>MKKIEHKMVAVNGLNMHLAELGEGPTILFIHGFPELWYSWRHQMVYLAERGYRAVAPDLRGYGDTTGAPLNDPSKFSILHLVGDVVALLEAIALNEEKVFVVAHDLGAYIAWHLCLFRPDKVKALVNLSVHFSKRNPKMNKVEGLKAIYGEDHYVSRFQVPGEIEAEFAPIGAKSVLKKILTYR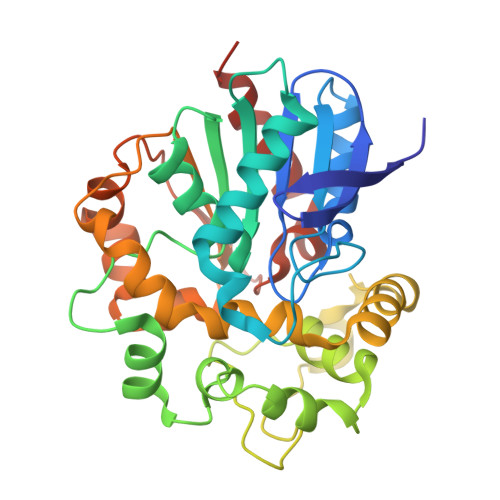DPAPLYFPKGKGLEAIPDAPVALSSWLSEEELDYYANKFEQTGFTGAVNYYRALPINWELTAPWTGAQVKVPTKFIVGEFDGVYHIPGAKEYIHNGGFKKDVPLLEEVVVLEGAAHFVSQERPHEISKHIYDFIQKFTSHHHHH[2x]>MGSSHHHHHHSSGRENLYFQGDIPQQLVERLQEEKRIEAQKRKERQEAHLYMQVQIVAEDQFCGHQGNDMYDEEKVKYTVFKVLKNSSL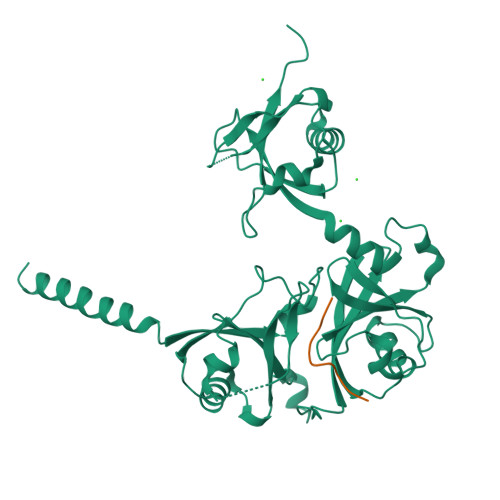AEFVQSLSQTMGFPQDQIRLWPMQARSNGTKRPAMLDNEADGNKTMIELSDNENPWTIFLETVDPELAASGATLPKFDKDHDVMLFLKMYDPKTRSLNYCGHIYTPISCKIRDLLPVMCDRAGFIQDTSLILYEEVKPNLTERIQDYDVSLDKALDELMDGDIIVFQKDDPENDNSELPTAKEYFRDLYHRVDVIFCDKTIPNDPGFVVTLSNRMNYFQVAKTVAQRLNTDPMLLQFFKSQGYRDGPGNPLRHNYEGTLRDLLQFFKPRQPKKLYYQQLKMKITDF[2x];>[2x]GPRKCARKTRH>[4x]LPAMEIECRITGTLNGVEFELVGGGEGTPEQGRMTNKMKSTKGALTFSPYLLSHVMGYGFYHFGTYPSGYENPFLHAINNGGYTNTRIEKYEDGGVLHVSFSYRYEAGRVIGDFKV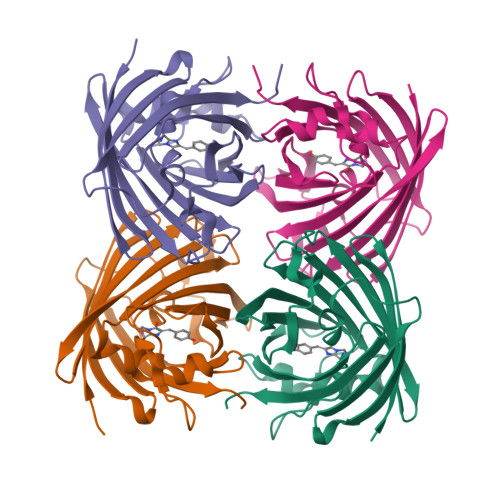MGTGFPEDSVIFTDKIIRSNATVEHLHPMGDNDLDGSFTRTFSLRDGGYYSSVVDSHMHFKSAIHPSILQNGGPMFAFRRVEEDHSNTELGIVEYQHAFKTPD> MASVHGTTYELLRRQGIDTVFGNPGSNELPFLKDFPEDFRYILALQEACVVGIADGYAQASRKPAFINLLSAAGTGNAMGALSNAWNSHSPLIVTAGQQTRAMIGVEALLTNVDAANLPRPLVKWSYEPASAAEVPHAMSRAIHMASMAPQGPVYLSVPYDDWDKDADPQSHHLFDRHVSSSVRLNDQDLDILVKALNSASNPAIVLGPDVDAANANADCVMLAERLKAPVWVAPSAPRCPFPTRHPCFRGLMPAGI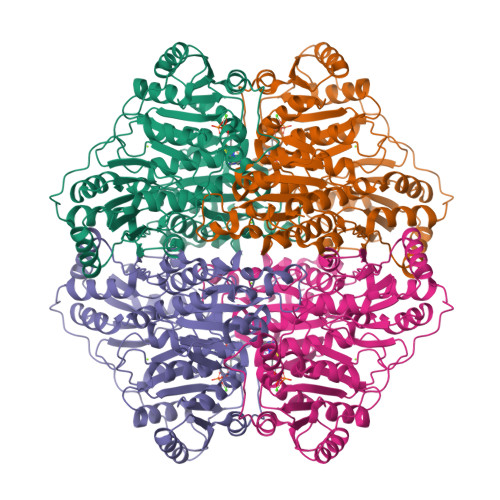AAISQLLEGHDVVLVIGAPVFRYHQYDPGQYLKPGTRLISVTCDPLEAARAPMGDAIVADIGAMASALANLVEESSRQLPTAAPEPAKVDQDAGRLHPETVFDTLNDMAPENAIYLNESTSTTAQMWQRLNMRNPGSYYFCAAGGLGFALPAAIGVQLAEPERQVIAVIGDGSANYSISALWTAAQYNIPTIFVIMNNGTYGALRWFAGVLEAENVPGLDVPGIDFRALAKGYGVQALKADNLEQLKGSLQEALSAKGPVLIEVSTVSPVKHHHHHH3,6,9,12,15,18-HEXAOXAICOSANE-1,20-DIOL | C14 H30 O8 | 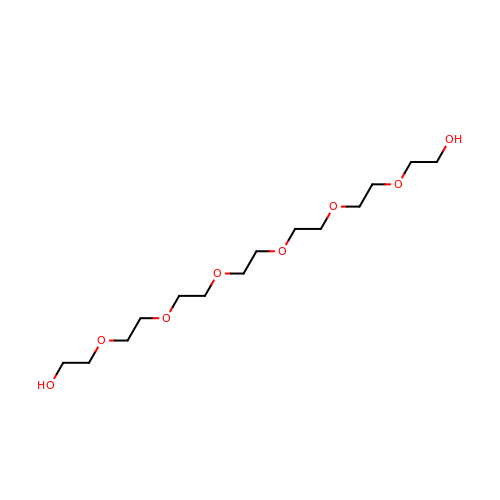XPJRQAIZZQMSCM-UHFFFAOYSA-N>MGSDKIHHHHHHMSSSQQIAKNARKAGNILKTISNEGRSDILYKIHDALKANAHAIEEANKIDLAVAKETGLADSLLKRLDLFKGDKFEVMLQGIKDVAELEDPVGKVKMARELDDGLTLYQVTAPVGVLLVIFESRPEVIANITALSIKSGNAAILKGGKESVNTFREMAKIVNDTIAQFQSETGVPVGSVQLIETRQDVSDLLDQDEYIDLVVPRGSNALVRKIKDTTKIPVLGHADGICSIYLDEDADLIKAKRISLDAKTNYPAGCNAMETLLINPKFSKWWEVLENLTLEGGVTIHATKDLKTAYFDKLNELGKLTEAIQCKTVDADEEQDFDKEFLSLDLAAKFVTSTESAIQHINTHSSRHTDAIVTENKANAEKFMKGVDSS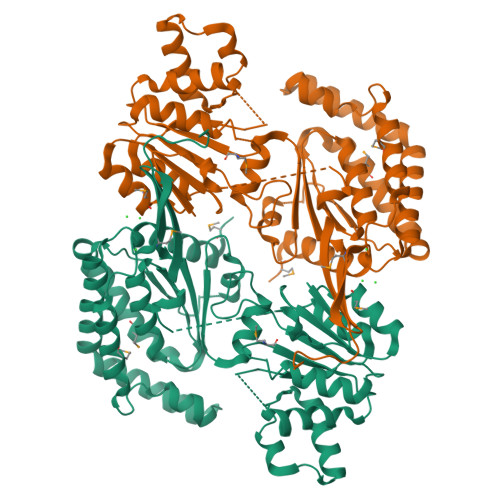GVYWNASTRFADGFRYGFGAEVGISTSKIHARGPVGLDGLVSYQYQIRGDGQVASDYLGAGGNKAFVHKDLDIKTVTL[2x]>SSSSESLSIIDVASDQNLFQTFIKEWRCKKRFSISLACEKIRSLTSSKTATIGSRFKQASSPQEIPIRDDGFPIKGCDDTLVVGLAVCWGGRDAYYFSLQKEQKHSEISASLVPPSLDPSLTLKDRMWYLQSCLRKESDKECSVVIYDFIQSYKILLLSCGISLEQSYEDPKVACWLLDPDSQEPTLHSIVTSFLPHELPLLEGMETSQGIQSLGLNAGSEHSGRYRASVESILIFNSMNQLNSLLQKENLQDVFRKVEMPSQYCLALLELNGIGFSTAECESQKHIMQAKLDAIETQAYQLAGHSFSFTSSDDIAEVLFLELKLPPNREMKNQGSKKTLGSTRRGIDNGRKLRLGRQFSTSKDVLNKLKALHPLPGLILEWRRITNAITKVVFPLQREKCLNPFLGMERIYPVSQSHTATGRITFTEPNIQNVPRDFEIKMPTLVGESPPSQAVGKGLLPMGRGKYKKGFSVNPRCQAQMEERAADRGMPFSISMRHAFVPFPGGSILAADYSQLELRILAHLSHDRRLIQVLNTGADVFRSIAAEWKMIEPESVGDDLRQQAKQICYGIIYGMGAKSLGEQMGIKENDAACYIDSFKSRYTGINQFMTETVKNCKRDGFVQTILGRRRYLPGIKDNNPYRKAHAERQAINTIVQGSAADIVKIATVNIQKQLETFHSTFKSHGHREGMLQSDQTGLSRKRKLQGMFCP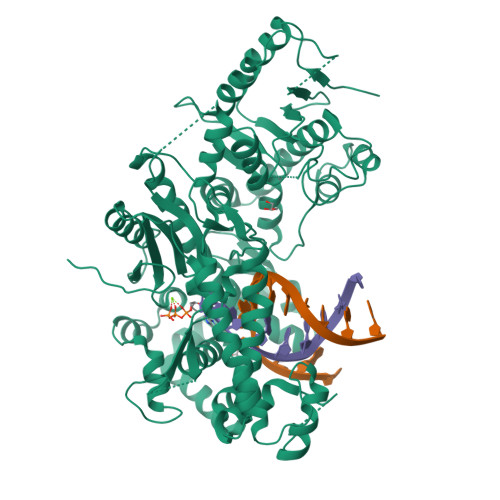IRGGFFILQLHDELLYEVAEEDVVQVAQIVKNEMESAVKLSVKLKVKVKIGASWGELKDFDV[2x]> MASPALQTCWRNLARLSGAQVRPSHFGAFSLGSRMSPFSSLLGARASPIATGRAGLRFLSSAAPNPGKKPASAAPPAGTNHGRITQVIGAVVDVHFDEQLPPILNSLEVQGHTNRLVLEVAQHLGENTVRTIAMDATEGLVRGQKVVDTGAPIQVPVGVETLGRIMNVIGEPVDECGPVPAKKTYSIHRAAPLFADQSTEPGLLQTGIKVVDLLAPYAKGGKIGLFGGAGVGKTVLIMELINNVANKHGGFSVFAGVGERTREGNDLYHEMMTTGVIKRKKLEDGKFDFTGSKAALVYGQMNEPPGARARVALTALSVAEYFRDE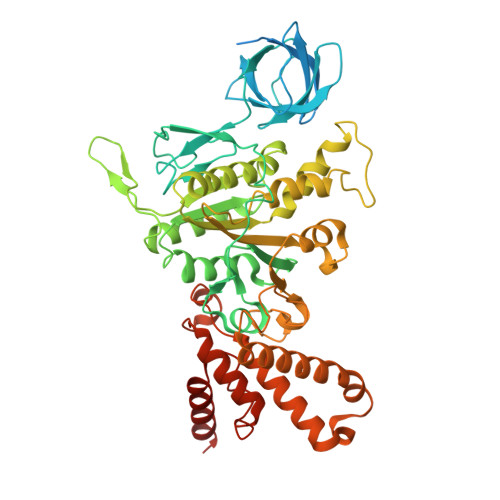QGQDVLLFIDNIYRFTQAGSEVSALLGRIPSAVGYQPTLATDLGQLQERITTTKKGSITSVQAVYVPADDLTDPAPATTFAHLDATTVLSRQIAELGIYPAVDPLDSTSRMLAPEIVGQEHYDTARATQKLLQDYKSLQDIIAILGMDELSEEDKLVVSRARKIQRFLSQPFTVAEVFTGKPGRFVELPETIKSAQTILRGECDDLPEMAFYMCGGLEEVRSKAVKMAQEAASGK> GAMGMESLFPNKGEIIRELLKDPLILKNDSKRSNGSELELDSSDLLQREAILANELNILDNLKTFLNLIKEVKTNLNILELENCYYSLQSLRKKMRNNAAYLKQSFNFQQSISTYVDTLHLELVSTLYKILTNGFWKITENSIQFTPTVEWGKDKVHIEYDTFMDFVAQQYFPKGSLDNQAWFILDMTSADSQEQVRAKLNTIMKEYMNLSRIVSMIKNSIFISGKEISYENEKNILVFSKSSSHGQHCVSTVLTSFEAVCDFMLDGLAFRDRKTLSYELGPL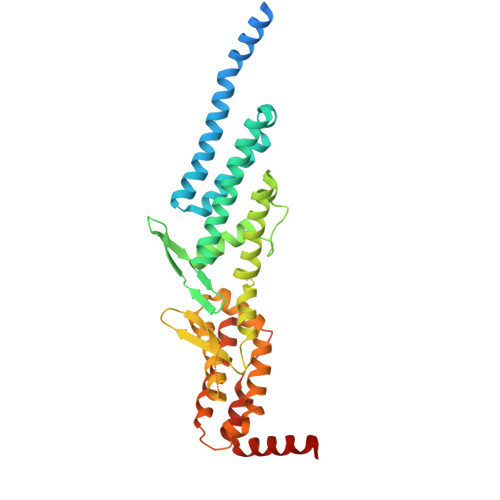FNTEFTKFVKNNASIILESLDSPLKNLVSVINNKLTRLVAKSEVTNWTHSGKEIQDLLMNKQLYYNLLLDKVLESHISEIRS>[2x]MARTVVLITGCSSGIGLHLAVRLASDPSQSFKVYATLRDLKTQGRLWEAARALACPPGSLETLQLDVRDSKSVAAARERVTEGRVDVLVCNA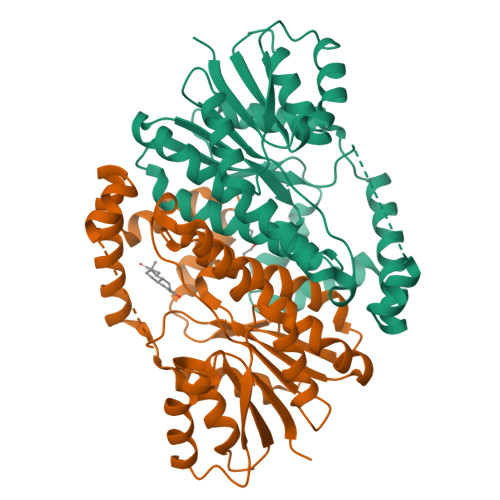GLGLLGPLEALGEDAVASVLDVNVVGTVRMLQAFLPDMKRRGSGRVLVTGSVGGLMGLPFNDVYCASKFALEGLCESLAVLLLPFGVHLSLIECGPVHTAFMEKVLGSPEEVLDRTDIHTFHRFYQYLAHSKQVFREAAQNPEEVAEVFLTALRAPKPTLRYFTTERFLPLLRMRLDDPSGSNYVTAMHREVFGDVPAKAEAGAEAGGGAGPGAEDEAGRGAVGDPELGDPPAAPQ> 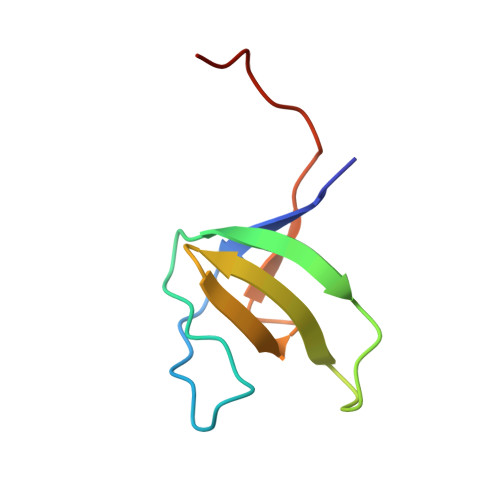ASDYCKVIFPYEAQNDDELTIKEGDIVTLINKDCIDVGWWEGELNGRRGVFPDNFVKLLPPLEHHHHHH>[4x]MNPPTTTTTTTRTIRAPKVQLTPNSATRRRRNRRRRRPAAAIAGPLSIQPSSINRRMVSRVTRRSAVVTAAGLAWLRQYLNPMGPDTTSVTGYPDGSAVTTCIADYSNTFNVSFPPREALYCTGSSSSEKPTLVDADNYAKIDKWSNYDITLCVLALPMLRNVVMLRLYPHTPTAFALTEQTPNFPQRFPNWSVYSADGTRFNNGD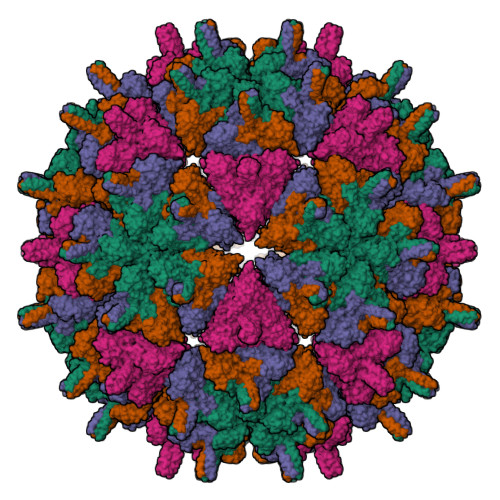EPGYLQSYVYLPNVDKHLSAARGYRLLSRGITGIFSAPALETQGFVTACQYLAEGSIQSQSIKSDAVRSVTVNSDGTVKNVESSSQTVSSMPRYVFPLDGDNCAPSSLTETYHQAYQSKATDGFYMPVLSSSRDNPFHPPQPRAIAVYGSFLARGCLDPVSEAHEADGPTHDIYRLNVADDVAPLFNTGVVWFEGISPKFSLKLKTRTVLQYIPTSGSVLANFTRHEPTYDQIALDAADRLRNLMPHAYPAAYNDWGWLGDLLDSAISMLPGVGTVYNIAKPLIKPAWNWLGNKVSDFFGNPVARDGDIFFDAK> MSGGDGRGHNTGAHSTSGNINGGPTGIGVSGGCSDGSGWSSENNPWGGGSG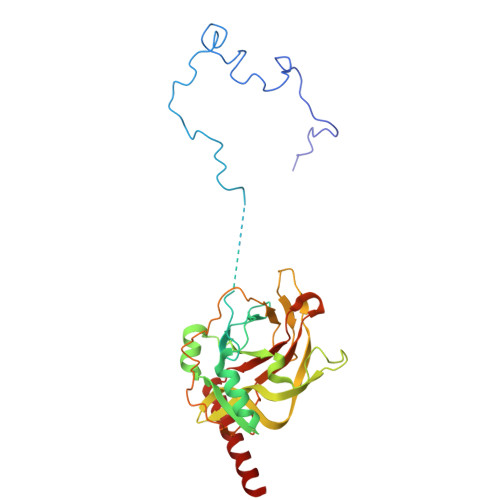SGIHWGGGSGRGNGGGNGNSGGGSGTGGNLSAVAAPVAFGFPALSTPGAGGLAVSISASELSAAIAGIIAKLKKVNLKFTPFGVVLSSLIPSEIAKDDPNMMSKIVTSLPADDITESPVSSLPLDKATVNVNVRVVDDVKDERQNISVVSGVPMSVPVVDAKPTERPGVFTASIPGAPVLNISVNDSTPAVQTLSPGVTNNTDKDVRPAGFTQGGNTRDAVIRFPKDSGHNAVYVSVSDVLSPDQVKQRQDEENRRQQEWDAT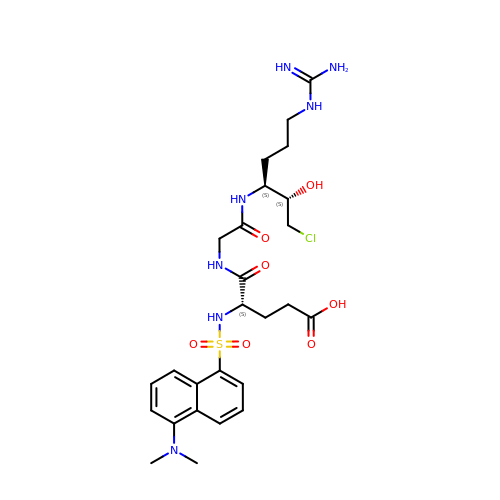N-{[5-(dimethylamino)naphthalen-1-yl]sulfonyl}-L-alpha-glutamyl-N-[(2S,3S)-6-carbamimidamido-1-chloro-2-hydroxyhexan-3-yl]glycinamide | C26 H38 Cl N7 O7 S | AKFRXQNHCCSRJN-IRFCIJBXSA-N> MVKSKAALLKKFSEPLSIEDVNIPEPQGEEVLIRIGGAGVCRTDLRVWKGVEAKQGFRLPIILGHENAGTIVEVGELAK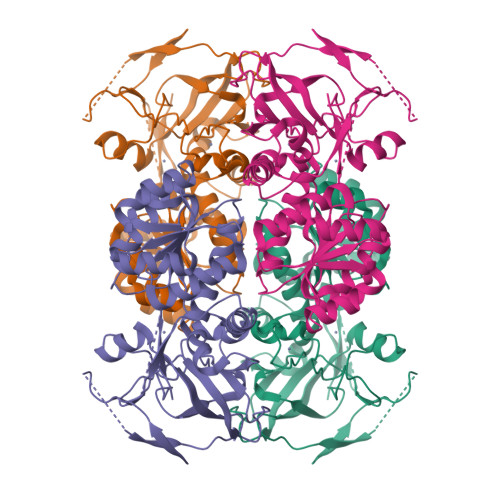VKKGDNVVVYATWGDLTCRYCREGKFNICKNQIIPGQTTNGGFSEYMLVKSSRWLVKLNSLSPVEAAPLADAGTTSMGAIRQALPFISKFAEPVVIVNGIGGLAVYTIQILKALMKNITIVGISRSKKHRDFALELGADYVSEMKDAESLINKLTDGLGASIAIDLVGTEETTYNLGKLLAQEGAIILVGMEGKRVSLEAFDTAVWNKKLLGSNYGSLNDLEDVVRLSESGKIKPYIIKVPLDDINKAFTNLDEGRVDGRQVITP>[2x]SNAIRPTIGQQMETGDQRFGDLVFRQLAPNVWQHTSYLDMPGFGAVASNGLIVRDGGRVLVVDTAWTNDQTAQ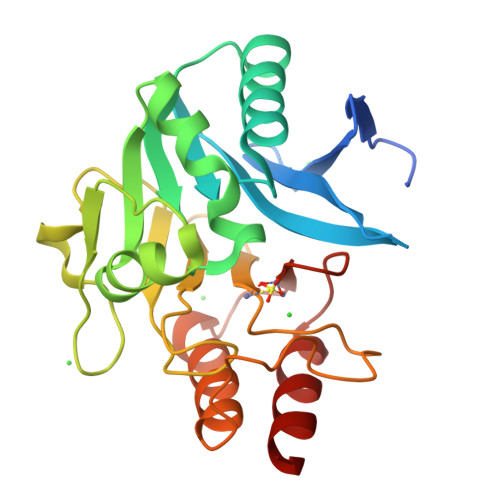ILNWIKQEINLPVALAVVTHAHQDKMGGMDALHAAGIATYANALSNQLAPQEGMVAAQHSLTFAANGWVEPATAPNFGPLKVFYPGPGHTSDNITVGIDGTDIAFGGCLIKDSKAKSLGNLGDADTEHYAASARAFGAAFPKASMIVMSHSAPDSRAAITHTARMADKLR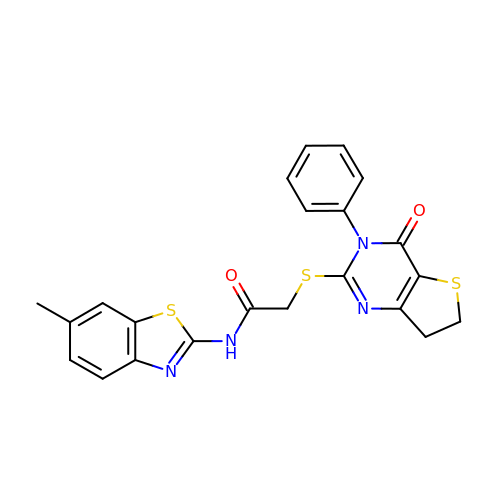~{N}-(6-methyl-1,3-benzothiazol-2-yl)-2-[(4-oxidanylidene-3-phenyl-6,7-dihydrothieno[3,2-d]pyrimidin-2-yl)sulfanyl]ethanamide | C22 H18 N4 O2 S3 | WRKPZSMRWPJJDH-UHFFFAOYSA-N>[2x]QTASPVIPTDPAIETHIREWL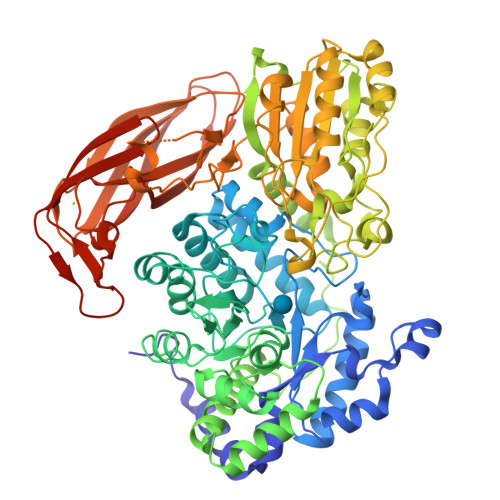QKMTLEQKIGQMCEITIDVVSDLETSRKKGFCLSEAMLDTVIGKYKVGSLLNVPLGVAQKKEKWAEAIKQIQEKSMKEIGIPCIYGVDQIHGTTYTLDGTMFPQGINMGATFNRELTRRGAKISAYETKAGCIPWTFAPVVDLGRDPRWARMWENYGEDCYVNAEMGVSAVKGFQGEDPNRIGEYNVAACMKHYMGYGVPVSGKDRTPSSISRSDMREKHFAPFLAAVRQGALSVMVNSGVDNGLPFHANRELLTEWLKEDLNWDGLIVTDWADINNLCTRDHIAATKKEAVKIVINAGIDMSMVPYEVSFCDYLKELVEEGEVSMERIDDAVARVLRLKYRLGLFDHPYWDIKKYDKFGSKEFAAVALQAAEESEVLLKNDGNILPIAKGKKILLTGPNANSMRCLNGGWSYSWQGHVADEYAQAYHTIYEALCEKYGKENIIYEPGVTYASYKNDNWWEENKPETEKPVAAAAQADIIITCIGENSYCETPGNLTDLTLSENQRNLVKALAATGKPIVLVLNQGRPRIINDIVPLAKAVVNIMLPSNYGGDALANLLAGDANFSGKMPFTYPRLINALATYDYKPCENMGQMGGNYNYDSVMDIQWPFGFGLSYTNYKYSNLKVNKPTFNADDELIFTVDVTNTGKVAGKESVLLFSKDLVASSTPDNIRLRNFEKVSLEPGETKTVTLKLKGSDLAFVGYDGKWRLEKGDFKIKCGDQWMDIVCDQTKVWNTPNKNTLHKLEHHHHHH>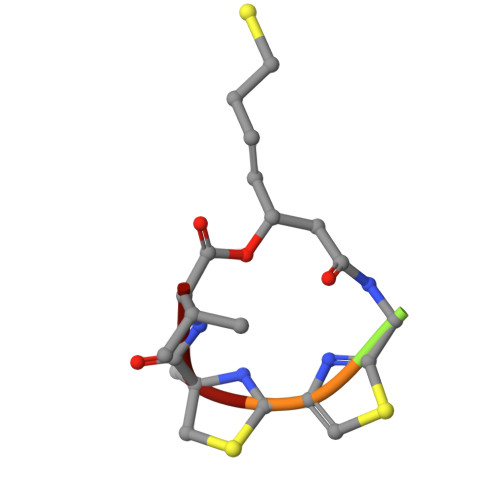 XGCCV>GSHMRDVVSFEQPEFSVSRGDQVARIPVIRRVLDGGKSQVSYRTQDGTAQGNRDYIPVEGELLFQPGEAWKELQVK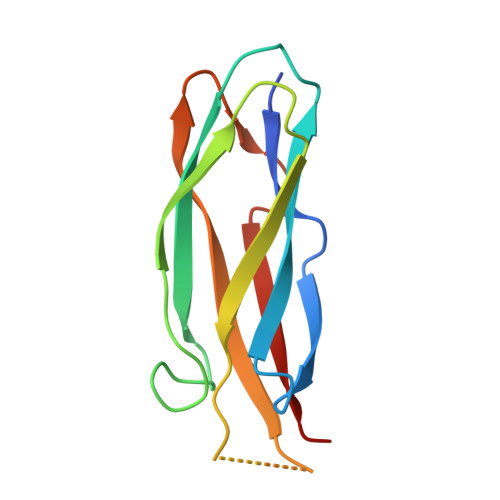LLELQEVDSLLRGRQVRRFHVQLSNPKFGAHLGQPHSTTIIIRDPDE[2x]> GSHMTIEQMVDRLLSYPERTKMQILAPIVSGKKGTHAKTLEDIRKQGYVRVRIDREMRELTGDIELEKNKKHSIDVVVDRIIIKDGIAARLADSLETALKLADGKVVVDVI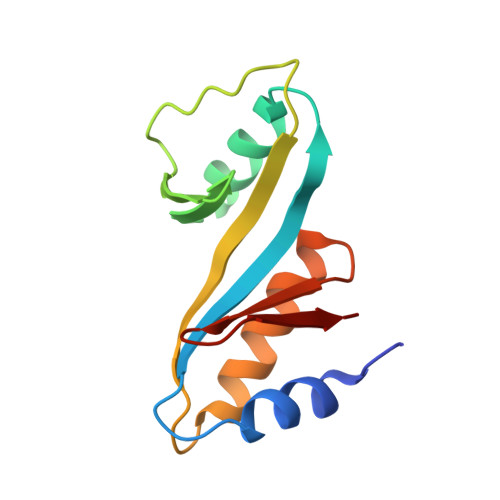GEGELLFS> MNLTELKNTPVSELITLGENMGLENLARMRKQDIIFAILKQHAKSGEDIFGDGVLEILQDGFGFLRSADSSYLAGPDDIYVSPSQIRRFNLRTGDTISGKIRPPKEGERYFA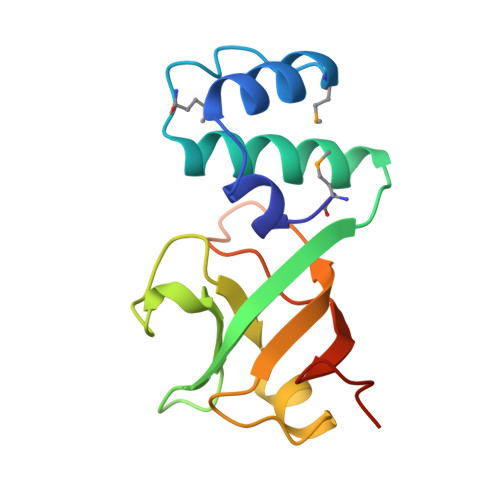LLKVNEVNFDKPENARNK> LGTNYLLSGQTLNTDGHLKNGDFDLVMQNDCNLVLYNGNWQSNTANNGRDCKLTLTDYGELVIKNGDGSTVWRS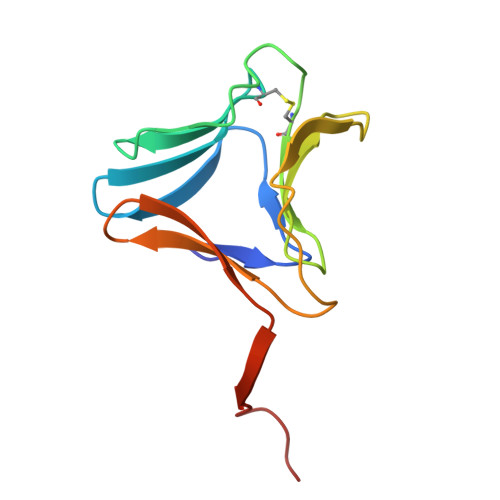RAKSVKGNYAAVLHPDGRLVVFGPSVFKIDPWVPGL>[2x]MGETTTIYMDIGDKKRTKGDFDGAIRAYKKVLKADPNNVETLLKLGKTYMDIGLPNDAIESLKKFVVLDTTSAEAYYILGSANFMIDEKQAAIDA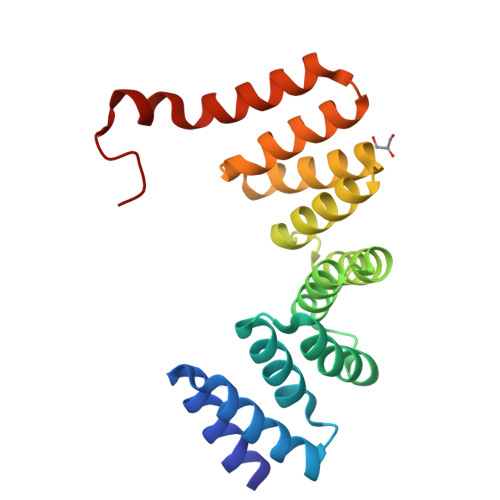LQRAIALNTVYADAYYKLGLVYDSMGEHDKAIEAYEKTISIKPGFIRAYQSIGLAYEGKGLRDEAVKYFKKALEKEEKKAKYELALVPR>[2x]MKIAIAGAGAMGSRFGLMLHQSGNEVLLIDGWAEHVQQIKEHGLQANFNGKEVEAKLPIVLQSE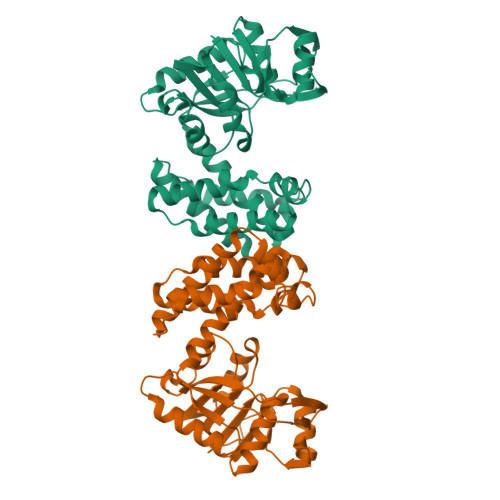VEKEDQVDLIILFTKAMQLEKMLQDIQSLIKKDTEVLCLLNGIGHEDIIEKFVPMENIYIGNTMWTAGLEGPGQVKLFGSGSVELQNLGDGKEAAAKKLADKLSESGLNAHFSDNIHYSIYRKACVNGTMNGLCTILDVNMAELGKTSTAHKMVATIVNEFAKVAAVEKIELDVPEVIAHCESCFDPETIGLHYPSMYQDLIKNHRLTEIDYINGAISRKGKKYGVATPYCDFLTELVHAKEDSLNVK>GHMSVTVPDKDWTLSSLSETFDDGTQTLQG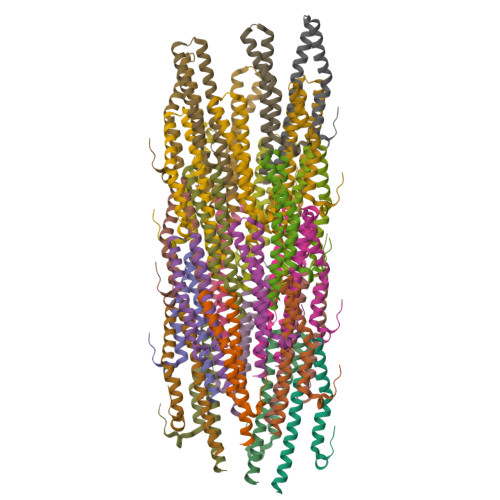QLTSALNALAENPSNPQLLAEYQSKLSEYTLYRNAQSNTVKVIKDVDAAIIQNFR[29x]> MIVIFVDFDYFFAQVEEVLNPQYKGKPLVVCVYSGRTKTSGAVATANYEARKLGVKAGMPIIKAMQIAPSAIYVPMRKPIYEAFSNRIMNLLNKHADKIEVASIDEAYLDVTNKVEGNFENGIELARKIKQEILEKEKITVTVGVAPNKILAKIIADKSKPNGLGVIRPTEVQDFLNELDIDEIPGIGSVLARRLNELGIQKLRDILSKNYNELEKITGKAKALYLLKLAQNKYSEPVENKSKIPHGRIVTMKRNSRNLEEIKPYLFRAIEESYYKLDKRIPKAIHVVAVTEDLDIVSRGRTFPHGISKETAYSESVKLLQKILEEDERKIRRIGVRFSK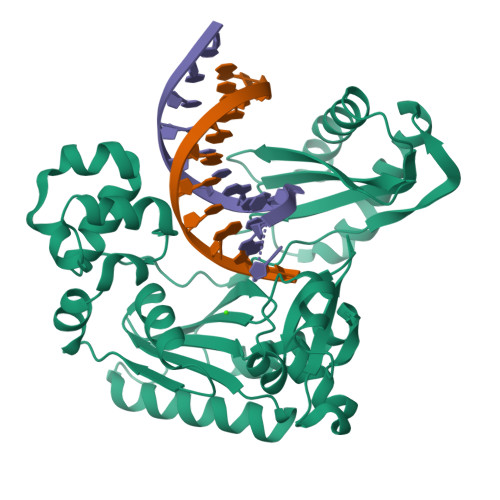FIEAIGLDKFFDTGGHHHHHH 3-{5-[(4aR,8aS)-3-cycloheptyl-4-oxo-3,4,4a,5,8,8a-hexahydrophthalazin-1-yl]-2-methoxyphenyl}prop-2-ynamide 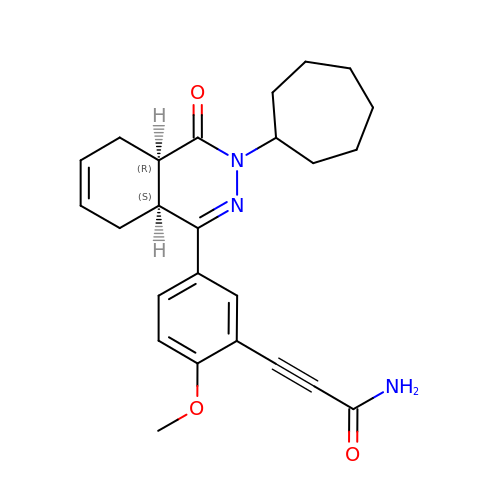| C25 H29 N3 O3 | YALZXZYFCQHHIY-LEWJYISDSA-N Evasins are chemokine-binding proteins from tick saliva, whose application as anti-inflammatory therapeutics will require manipulation of their chemokine target selectivity. Here we describe subclass A3 evasins, which are unique to the tick genus Amblyomma and distinguished from “classical” class A1 evasins by an additional disulfide bond near the chemokine recognition interface. The A3 evasin EVA-AAM1001 (EVA-A) bound to CC chemokines and inhibited their receptor activation. Structures of chemokine-bound EVA-A revealed a deep hydrophobic pocket, unique to A3 evasins, that interacts with the residue immediately following the CC motif of the chemokine.

In the EVA-A:chemokine structures, the side chain of the chemokine CC + 1 residue (Tyr in CCL7; Phe in CCL11, Leu in CCL16 and CCL17) sits in a deep hydrophobic pocket within the evasin structure, possibly enabling the ~35° rotation of the chemokine relative to its position in class A1 evasin complexes. Notably, this “CC + 1 recognition pocket” is defined by several hydrophobic side chains and by the Cys22-Cys51 disulfide bond, the fifth disulfide that distinguishes class A3 from class A1 evasins (Fig. 3a expansion). Moreover, we found that mutation of Cys22 and Cys51 to Ser, giving EVA-A(C8), resulted in significantly or substantially diminished binding affinity (or loss of measurable binding) to most chemokines. Nevertheless, this double mutant co-crystallised with CCL17, with the only structural changes being in the immediate vicinity of the mutated disulfide bond. Thus, it appears that the key function of the unique disulfide bond in class A3 evasins is to structurally define the CC + 1 recognition pocket. Second, the additional disulfide bond of class A3 evasins enables the formation of a deep hydrophobic pocket for binding to the chemokine CC + 1 residue. EVA-A accommodates this residue within a hydrophobic pocket, which is formed by the disulfide bond that defines class A3 evasins as well as the side chains of residues Leu39, Tyr44 and Tyr57.

> GSTSARNHTEDNSTEYYDYEEARSACPARHLNNTNGTVLKLLGCHYFCNGTLSTAPDGYPCYNLTAQQVRTLTTYPNTSCAVGVCMKGTCVKNGTMEQCFKTP;> ARGTNVGRECCLEYFKGAIPLRKLKTWYQTSEDCSRDAIVFVTVQGRAICSDPNNKRVKNAVKYLQSLERS> MKLYYTPGSCSLSPHIVLRETGLDFSIERIDLRTKKTESGKDFLAINPKGQVPVLQLDNGDILTEGVAIVQYLADLKPDRNLIAPPKALERYHQIEWLNFLASEVHKGYSPLFSSDTPESYLPVVKNKLKSKFVYINDVLSKQKCVCGDHFTVAD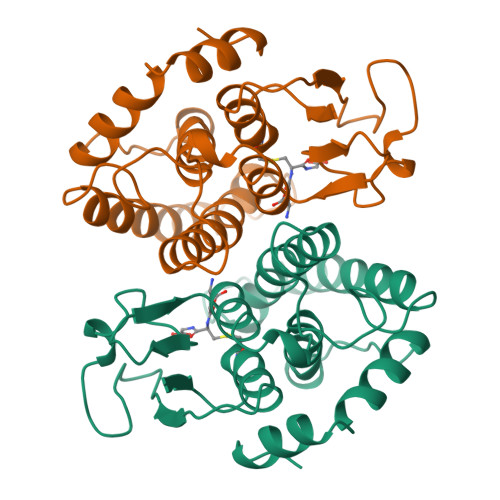AYLFTLSQWAPHVALDLTDLSHLQDYLARIAQRPNVHSALVTEGLIKE>[4x]MFNRIMVPVDGSKGAVKALEKGVGLQQLTGAELYILCVFKHHSLLEASLSMARPEQLDIPDDAL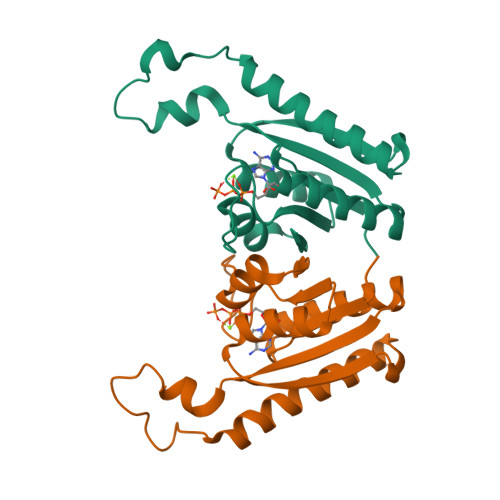KDYATEIAVQAKTRATELGVPADKVRAFVKGGRPSRTIVRFARKRECDLVVIGAQGTNGDKSLLLGSVAQRVAGSAHCPVLVV>[4x]SLKGKIEWVRVSAVVHSTEDREKVGEAISTLFPFEFEIAVSKAKGHYGNPMEYLEVELTKSSEIKKFWKNLLELLGEQAEEILSTLEDRIDEQNVLHIRIDKQKAYLGEVSLTSGGDPIAVKLRLVTYPSKREKVIEFARELCTIS

UPF0201 family proteins constitute one such uncharacterized, archaeal specific protein family. The UPF0201 family proteins occur as a single globular α/β domain with approximate dimensions of 55×35×35 Å3. The protomeric structure consists of a five-stranded, anti-parallel β-sheet, five α helices, which are located on one face of the β-sheet, and three loops connecting helices and strands. We have further documented that all members of this archaeal specific protein family share a common polypeptide chain fold, which is evolutionarily related to the RRM motif found in the ribosomal L5 proteins and many other RNA-binding proteins.

For 10077d from A. fulgidus, the N-terminal His6 tagged full length protein gave crystals and a structure, whereas the C-terminal His6 tagged version yielded neither. In none of the three X-ray structures of full-length UPF0201 proteins was electron density corresponding to the 15–20 C-terminal residues observed. The loop connecting β2 and β3 protrudes somewhat from the globular domain, and the electron density corresponding to this region is poorly defined in the 10077b and 10077d structures. Our four UPF0201 structures represent subfamilies N149845 (10077a, b) and N130963 (10077c, d). The crystallographic asymmetric units contain one protomer in 10077c, two in 10077b and four protomers in both 10077a and 10077d. While 10077a, 10077b and 10077d all form one type of dimer (typeI), 10077c forms altogether different dimer via crystallographic symmetry (typeII). The interface surface area for type I dimers in 10077a, 10077b and 10077d are 672, 563 and 611 Å2, respectively.2-(6-hydroxy-3-oxo-3H-xanthen-9-yl)-5-[(E)-(sulfanylmethylidene)amino]benzoic 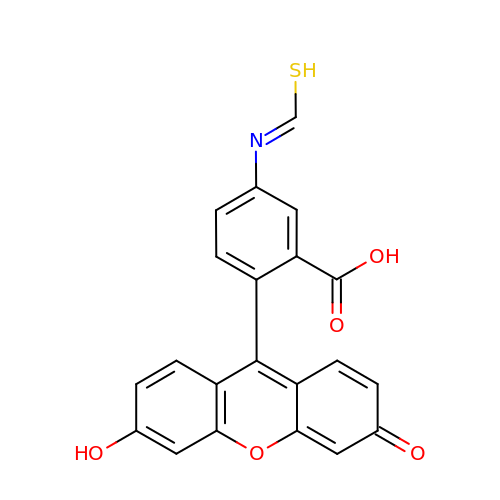acid | C21 H13 N O5 S | KDFRZGWCOSXMPY-UHFFFAOYSA-N> SVQQASRSKVSVAPLHLESAKEPPLNTYKPKEPFTATIVSVESLVGPKAPGETCHIVIDHGGNVPYWEGQSYGVIPPGEN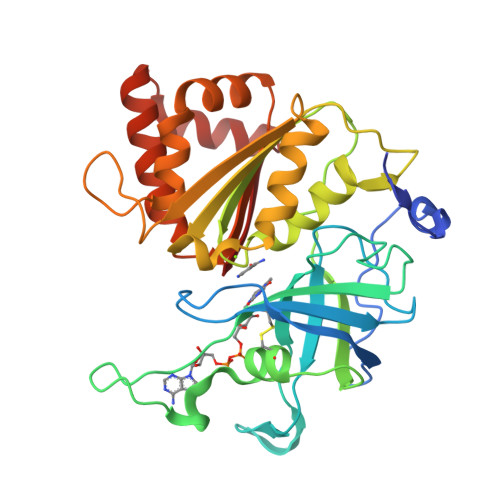PKKPGAPQNVRLYSIASTRYGDNFDGRTGSLCVRRAVYYDPETGKEDPSKNGVCSNFLCNSKPGDKIQLTGPSGKIMLLPEEDPNATHIMIATGTGVAPFRGYLRRMFMEDVPNYRFGGLAWLFLGVANSDSLLYDEEFTSYLKQYPDNFRYDKALSREQKNRSGGKMYVQDKIEEYSDEIFKLLDGGAHIYFCGLKGMMPGIQDTLKKVAERRGESWDQKLAQLKKNKQWHVEVA> MLNIGDLLGSTPAKDQACSRTCESQFCTIAPLLRYGKYCGILYSGCPGERPCDALDACCMVHDHCVDTHNDDYLNTMCNENLLSCIDRVSGATFPGNKCNVGQTASVIRGVIETAVFAGKILHKRDDGQ;>MLNIGDLLGSTPAKDQGCSRTCESQFCTIAPLLRYGKYCGILYSGC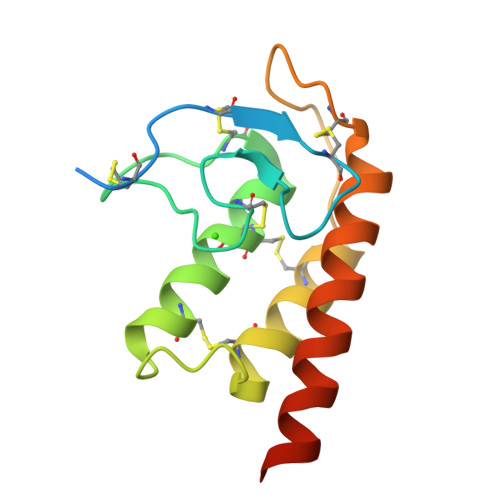PGERPCDALDACCMVHDHCVDTHNDDYLNTMCNENLLSCIDRVSGATFPGNKCNVGQTASVIRGVIETAVFAGKILHKRDDGQ[2x]> ASAKLPGDFGPPRGEPIHAVLTSPPLVPPPVNRTYPAKVIVELEVVEKEMQISEGVSYTFWTFGGTVPGSFIRVRQGDTVEFHLKNHPSSKMPHNINLHGVTGPGGGAASSFTAPGHESQFTFKALNEGIYVYHCATAPVGMHIANGMYGLILVEPPEGLP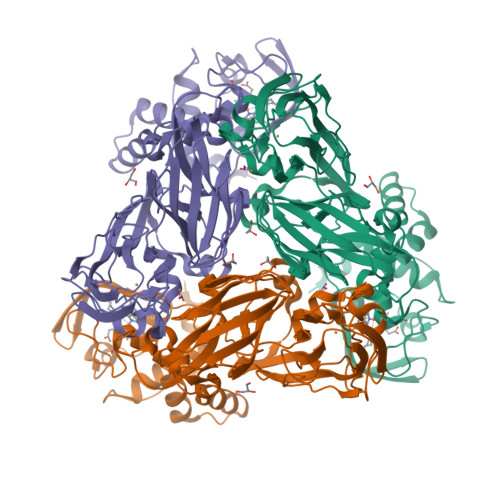KVDHEYYVMQGDFYTAGKYREKGLQPFDMEKAIDERPSYVLFNGAEGALTGDKALHAKVGETVRIFVGNGGPNLVSSFHVIGAIFDQVRYEGGTNVQKNVQTTLIPAGGAAVVKFTARVPGSYVLVDHSIFRAFNKGAMAILKIDGAENKLVYSGKELDSVYLGDRAAPNMSAVTKATQASVSGTLTVQDQVQAGRALFAGTCSVCHQGNGAGLPGVFPPLAKSDFLAADPKRAMNIVLHGLNGKIKVNGQEYDSVMPPMTQLNDDEVANILTYVLNSWDNPGGRVSAEDVKKVRAQPAPAKAVAEH> IVGGRRARPHAWPFMVSLQLRGGHFCGATLIAPNFVMSAAHCVANVNVRAVRVVLGAHNLSRREPTRQVFAVQRIFENGYDPVNLLNDIVILQLNGSATINANVQVAQLPAQGRRLGNGVQCLAMGWGLLGRNRGIASVLQELNVTVVTSLCRRSNVCTLVRGRQAGVCFGDSGSPLVCNGLIHGIASFVRGGCASGLYPDAFAPVAQ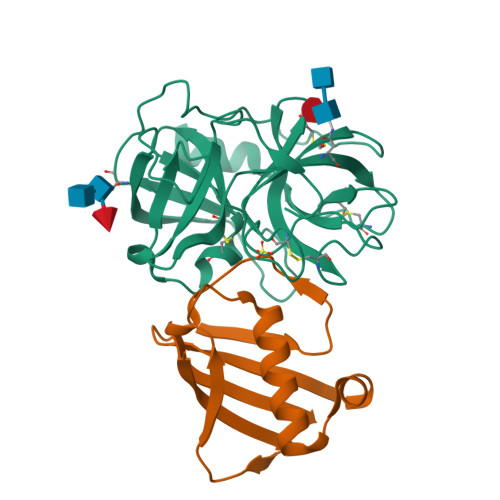FVNWIDSIIQ;> GSTRYVPYTIAVNGTSTPILSKLKISNKQLISYKYLNDKVKSVLKSERGISDLDLKFAKQAKYTVYFKNGKKQVVNLKSDIFTPNLFSAKDIKKIDIDVKQYTKSKKK>MQFPQLDPATLAAFSAAFRGELIWPSDADYDEARRIWNGTIDRRPALIARCTSTPDVVAAVSFARKSGLLVAVRGGGHSMAGHSVCDGGIVIDLSLMNSIKVSRRLRRARAQGGCLLGAFDTATQAHMLATPAGVVSHTGLGGMVLGGGFGWLSRKYGLSIDNLTSVEIVTADGGVLTASDTENPDLFWAVRGGGGNFGVVTAFEFDLHRVGPVRFASTYYSLDEGPQVIRAWRDHMATAPDELTWALYLRLAPPLPELPADMHGKPVICAMSCWIGDPHEGERQLESILHAGKPHGLTKATLPYRALQAYSFPGAVVPDRIYTKSGYLNELSDEATDTVLEHAADIASPFTQLELLYLGGAVARVPDDATAYPNRQSPFVTNLAAAWMDPTEDARHTAWAREGYRALAGHLSGGYVNFMNPGEADRTREAYGAAKFERLQGVKAKYDPTNLFRLNQNIPPSSP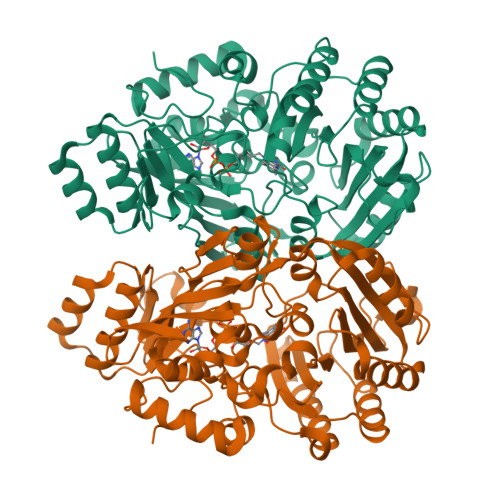[4x]> MIKVEIKPSQAQF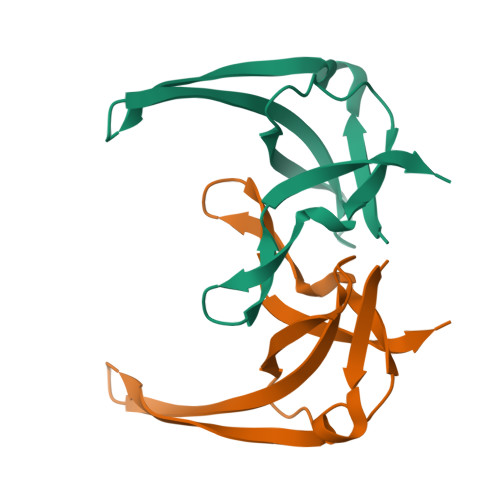TTRSGVSRQGKPYSLNEQLCYVDLGNEFPVLVKITLDEGQPAYAPGLYTVHLSSFKVGQFGSLMIDRLRLVPAK>[4x]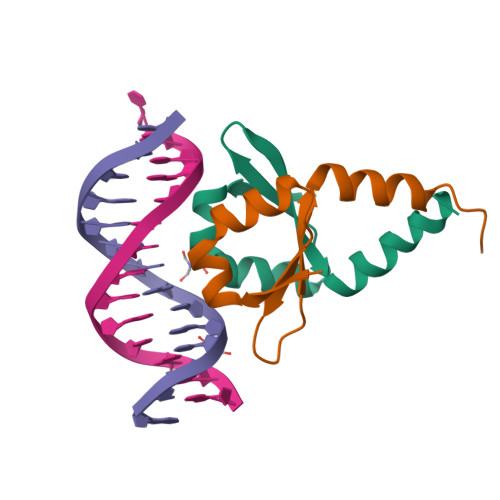MQSINFRTARGNLSEVLNNVEAGEEVEITRRGREPAVIVSKATFEAYKKAALDAEFASLFDTLDSTNKELVNR> ASIKENSYFAGGVKSLGFNQHGQDVSVGVMLPGEYTFGTQAPERMTVVKGALVVKRVGEADWTTYSSGESFDVEGNSSFELQVKDAT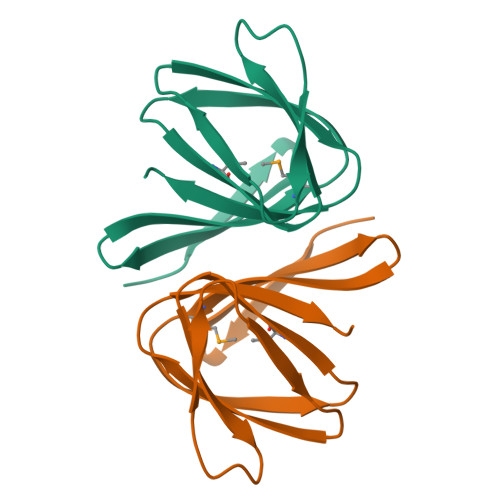AYLCEYL> 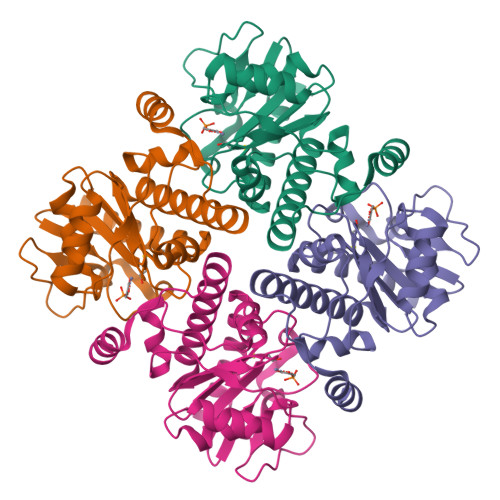MERNKLARQIIDTCLEMTRLGLNQGTAGNVSVRYQDGMLITPTGIPYEKLTESHIVFIDGNGKHEEGKLPSSQWRFHMAAYQSRPDANAVVHNHAVHCTAVSILNRSIPAIHFMIAAAGGNSIPCAPYATFGTRELSEHVALALKNRKATLLQHHGLIACEVNLEKALWLAHEVEVLAQLYLTTLAITDPVPVLSDEEIAVVLEKFKTFGLRIEE>MSLKLIGMLDSPYVRRVAISLKSLGLPFEHHSLSVFSTFEQFKAINPVVKAPTLVCEGGEVLMDSSLIIDYLETLAGPQRSLMPTALPQRLRELRLVGLALAACEKSVQIVYERNLRPAEKQHGPWLERVG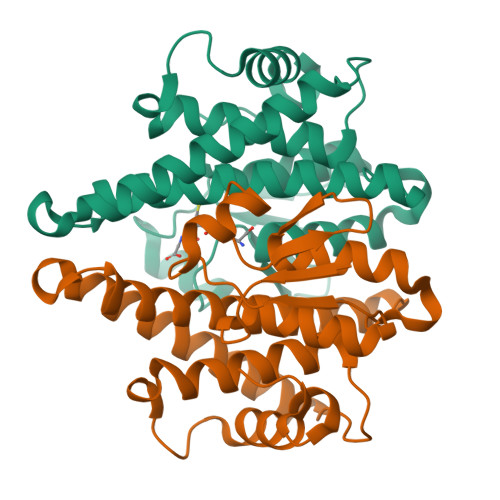GQLQAAYGELEQELQKQPLPRDGSLGQAGISLAVAWSFSQMMVADQFNPGQFPAVRGFAEYAEQLPVFLATPATEGHHHHHH[2x]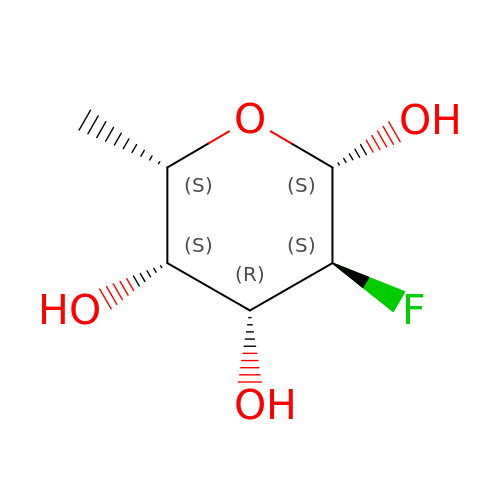2-deoxy-2-fluoro-beta-L-fucopyranose | C6 H11 F O4 | IRKXGKIPOMIQOD-QYESYBIKSA-N> GSMNQATQIIPFTTSGSLVDYVDRKVIVV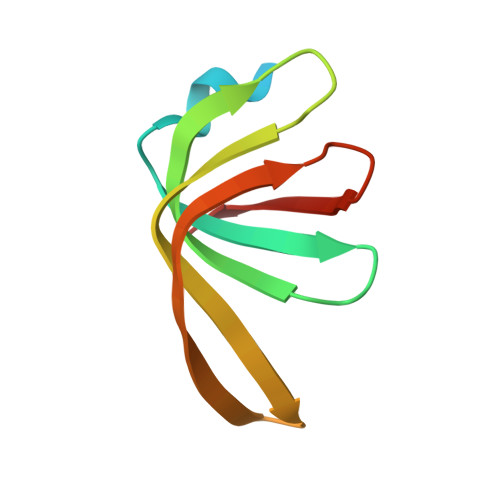LRDGKKLIGILRSFDQFANLMLQYTIERIYVDDMYGDIDRGVYIVRGENVVLLGELD> AARK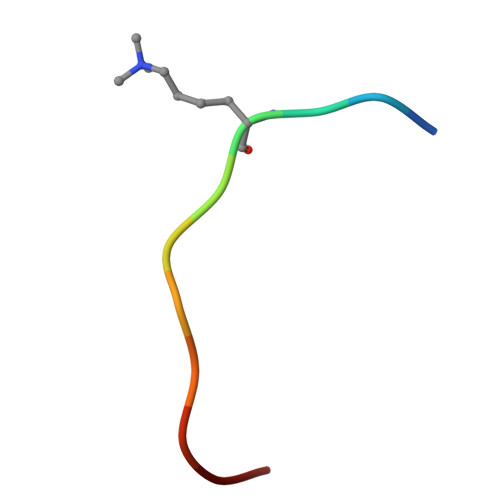SAPATGG>[2x]MKGEGVIVGILNKNFSLSKGDLDVVSLGEILVDMISTEEVNSLSQSREYTRHFGGSPANIAVNLSRLGKKVALISRLGADAFGNYLLDVLKGEQIITDGIQQDKERRTTIVYVSKSTRTPDWLPYREADMYLQEDDIIFELIKRSKVFHLSTFILSRKPARDTAIKAFNYAREQGKIVCFDPCYRKVLWPEGD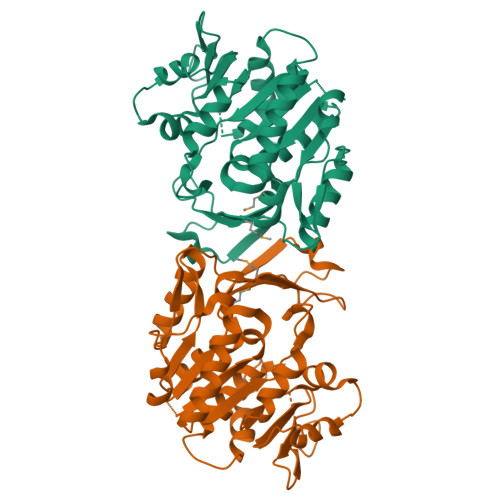DGAGVVEEIISRADFVKPSLDDARHLFGPDSPENYVKRYLELGVKAVILTLGEEGVIASDGEEIIRIPAFSEDAVDVTGAGDAFWSGFICGLLDGYTVKRSIKLGNGVAAFKIRGVGALSPVPSKEDIIKEYNI Ets-2, like its closely related homologue Ets-1, is a member of the Ets family of DNA binding transcription factors. Ets proteins share an 85-amino acid winged helix-turn-helix DNA binding domain (the Ets domain) that recognizes the conserved core DNA sequence GGA(A/T) through direct polar contacts mediated by residues in the highly conserved recognition helix (α3). Several of the Ets family members such as Ets-1, Ets-2, Etv-4, Etv-5, and Etv-6 are subject to autoinhibition in which additional structural elements outside of the core Ets domain inhibit DNA binding. Much of the knowledge of autoinhibition in Ets family proteins comes from studies on Ets-1, which is closely related to Ets-2 (84% sequence identity for the Ets domains and 55% across the entire length of the polypeptide) and, like Ets-2, contains 4 additional α-helices located immediately N-terminal (HI-1 and HI-2) and C-terminal (H4 and H5) to the core Ets domain.

Crystals of the Ets-2 DNA complex were obtained with an Ets-2 construct spanning residues 325–464, including the N-terminal (HI-1 and HI-2) and C-terminal (H4 and H5) autoinhibitory regions and the DNA oligonucleotides 5′-ACCGGAAGTG and 5′-CACTTCCGGT. The crystals belong to a primitive monoclinic crystal system, space group P 21, and diffracted to 2.5 Å resolution with 3 copies of Ets-2 and three 10-bp DNA duplexes in the asymmetric unit. An examination of the three Ets-2 molecules in the asymmetric unit reveals that, although they all share the same core Ets family fold and interact with double-stranded DNA in a similar manner, the autoinhibitory regions are significantly different, being well ordered in chain A but almost completely disordered in the other two chains (D and G). In chain A the entire autoinhibitory module can be seen to form a complete folded helical structure and associates with the core of the Ets domain via an extensive interface formed by H1 and the β1-β2 loop. The HI-1 helix, which was suggested to undergo a structural transition from ordered to disordered upon DNA binding, is well ordered and forms a helical secondary structure that packs against the C-terminal ends of helices H4 and HI-2, burying two predominant aromatic residues (Phe-331 and Tyr-334). For the remaining chains in the asymmetric unit (chain D and G) the entire autoinhibitory module was either completely or partially disordered and was not modeled in final structure. There are also a large number of side-chain residues that transition from being ordered in the autoinhibited form to being disordered in the other two chains; a significant proportion of these (Asp-387, Arg-401, Arg-406, Lys-436, and Arg-441) participate in intramolecular salt bridges in the autoinhibited form.

>SMNKPTMSFKDYIQERSDPVEQGKPVIPAAVLAGFTGSGPIQLWQFLLELLSDKSCQSFISWTGDGWEFKLADPDEVARRWGKRKNKPKMNYEKLSRGLRYYYDKNIIHKTSGKRYVYRFVCDLQNLLGFTPEELHAILGVQ[3x]> MTISTLSNETTKSGSCSGQGKNGGKDFTYGKKCFTKEEWKEQVAKYSAMGELYANKTIHYPLKIQPNSSGGSQDEGFATIQTTPIEPTLPRLLLNYFVSMAYEDSSIRMAKELGFIRNNKDIAVFNDLYKIKERF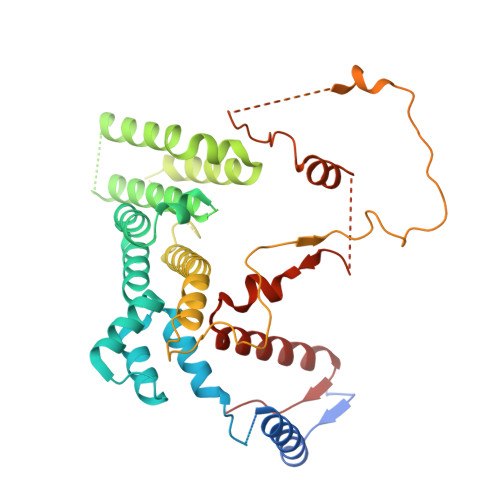HIKHLIKLGRINEAMEEINSIFGLEVLEETFNATGSYTGRTDRQQQQQQQQFDIDGDLHFKLLLLNLIEMIRSHHQQENITKDSNDFILNLIQYSQNKLAIKASSSVKKMQELELAMTLLLFPLSDSADSGSIKLPKSLQNLYSISLRSKIADLVNEKLLKFIHPRIQFEISNNNSKFPDLLNSDKKIITQNFTVYNNNLVNGSNGTKITHISSDQPINEKMSSNEVTAAANSVWLNQRDGNVGTGSAATTFHNLENKNYWNQTSELLSSSNGKEKGLEFNNYYSSEFPYEPRLTQIMKLWCWCENQLHHNQIGVPRVEN Recently, a shortened Dscam (sDscam) gene family with tandemly arrayed 5′ cassettes in Chelicerata species has been identified, which encodes ∼50–100 isoforms. Chelicerata sDscams could be classified into two subfamilies, sDscamα and sDscamβ, containing one and two variable Ig domains, respectively. Crystal structures and cell aggregation assays demonstrated that both α and β subfamilies of sDscam used Ig1 for the isoform-specific trans recognition in a hand-in-hand manner. Furthermore, the cis interactions were established by the three FNIII domains of sDscam, which assemble into a cross fold with a kink between FNIII2 and FNIII3.

We found that FNIII2 alone but not FNIII1 or FNIII3 could promote cKIT tyrosine phosphorylation, suggesting the essential role of FNIII2 domain in mediating sDscam cis interactions. The gel-filtration analysis supported our observations in the crystal structures: Ig1 mediated the formation of trans homodimer and all the three FNIII domains were involved in the cis interactions.

>[6x]GASPPLPSISISHVTSSSVQLNWENSQAVPASTIKQYLLEFRGDNKDWIKLHIPNNRKSFVLNGLDSSRRYQLRLAAYNRYGRGDFAVIGFTTAHKE> MAISRELVDPNSSPREIEVSEPREVGITELVLRDAHQSLMATRMAMEDMVGACADIDAAGYWSVECWGGATYDSCIRFLNEDPWERLRTFRKLMPNSRLQMLLR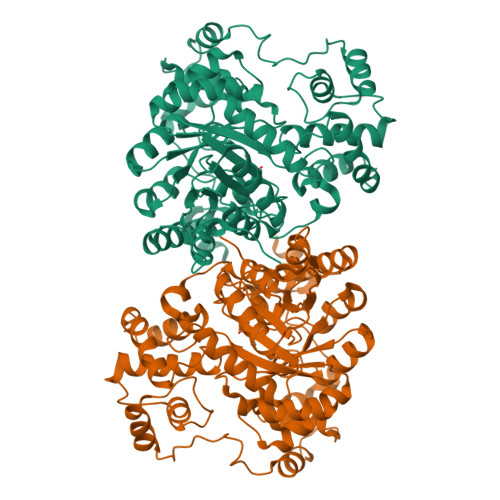GQNLLGYRHYNDEVVDRFVDKSAENGMDVFRVFDAMNDPRNMAHAMAAVKKAGKHAQGTICYTISPVHTVEGYVKLAGQLLDMGADSIALKDIAALLKPQPAYDIIKAIKDTYGQKTQINLHCHSTTGVTEVSLMKAIEAGVDVVDTAISSMSLGPGHNPTESVAEMLEGTGYTTNLDYDRLHKIRDHFKAIRPKYKKFESKTLVDTSIFKSQIPGGMLSNMESQLRAQGAEDKMDEVMAEVPRVRKAAGFPPLVTPSSQIVGTQAVFNVMMGEYKRMTGEFADIMLGYYGASPADRDPKVVKLAEEQSGKKPITQRPADLLPPEWEKQSKEAATLKGFNGTDEDVLTYALFPQVAPVFFEHRAEGPHSVALTDAQLKAEAEGDEKSLAVAGPVTYNVNVGGTVREVTVQQATRASQPELAPEDPEDLEHHHHHH> MGEQNNRPTDERIIDPSTANTQLTGGVCYNTTSGGNKPLAGSPYGYETWIDTGGGVCSLCWYGADQGGGAAFKATWTNPHDFLGRLGYFWNENKPYSHYENIYCGFNYTRSGR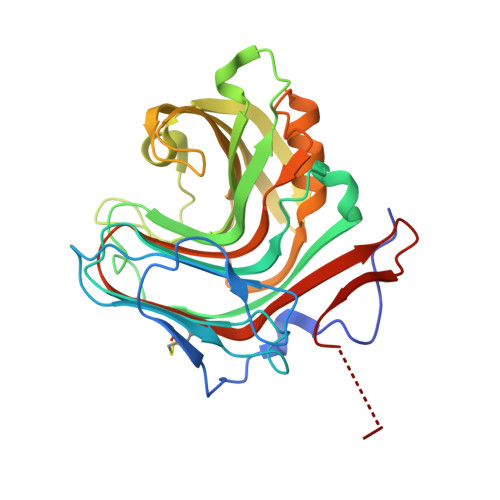KTAGDYSYIGIYGWSRNPSASNSNERLIEYYIVEDWFGNQWQADTSPMGINTTGGTVMGSFTVDGSSYQIIKNTRVNQPSIEGDKTFVQYFSIRQSPRKSGTISITEHFRKWERLGMKLGDNMYECKFLIEAGAGEGFFDARLIQFYRADNEGNILQITPLEHHHHHH>MHHHHHHMILLVSPIDVEEAKEAIAGGADIIDVKNPKEGSLGANFPWMIKAIREVTPKDLLVSATVGDVPYKPGTISLAAVGAAISGADYIKVGLYGVKNYYQAVELMKNVVRAVKDIDENKIVVAAGYADAYRVGAVEPLIVPKI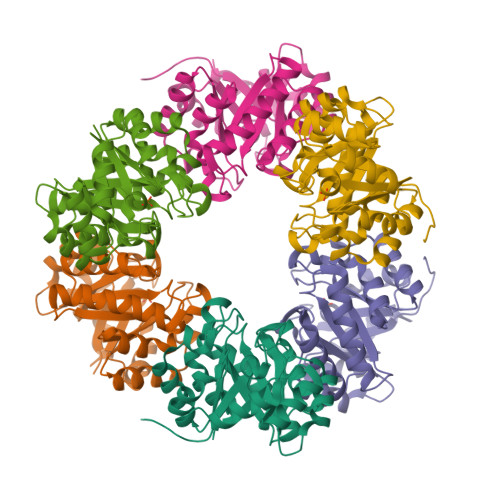ARDAGCDVAMLDTAIKDGKTLFDFQSKEILAEFVDEAHSYGLKCALAGSIKKEHIPILKEIGTDIVGVRGAACKGGDRNNGRIDRELVKELKELCK[9x]>MAAAAVSGALGRAGWRLLQLRCLPVARCRQALVPRAFHASAVGLRSSDEQKQQPPNSFSQQHSETQGAEKPDPESSHSPPRYTDQGGEEEEDYESEEQLQHRILTAALEFVPAHGWTAEAIAEGAQSLGLSSAAASMFGKDGSELILHFVTQCNTRLTRVLEEEQKLVQLGQAEKRKTDQFLRDAVETRLRMLIPYIEHWPRALSILMLPHNIPSSLSLLTSMVDDMWHYAGDQSTDFNWYTRRAMLAAIYNTTELVMMQDSSPDFEDTWRFLENRVNDAMNMGHTAKQVKSTGEALVQGLMGAAVTLKNLTGLNQRR[4x];>[4x]MSCAGAAAAPRLWRLRPGARRSLSAYGRRTSVRFRSSGMTLDNISRAAVDRIIRVDHAGEYGANRIYAGQMAVLGRTSVGPVIQKMWDQEKDHLKKFNELMVTFRVRPTVLMPLWNVLGFALGAGTALLGKEGAMACTVAVEESIAHHYNNQIRTLMEEDPEKYEELLQLIKKFRDEE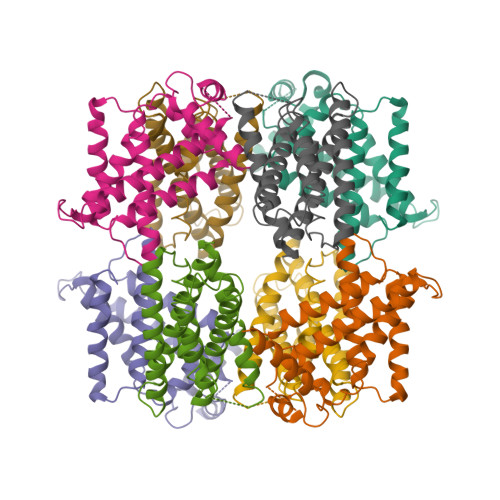LEHHDIGLDHDAELAPAYAVLKSIIQAGCRVAIYLSERL> SDKIIHLTDDSFDTDVLKADGAILVDFWAEWCGPCKMIAPILDEIADEYQGKLTVAKLNIDQNPGTAPKYGIRGIPTLLLFKN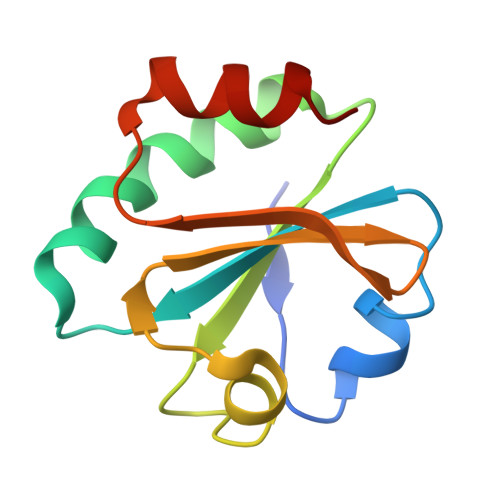GEVAATKVGALSKGQLKEFLDANLA>MSQSGEDLHSPTYLSWRKLQLSRAKLKASSKTSALLSGFAMVAMVEVQLDHDTNVPPGMLIAFAICTTLLVAVHMLALMISTCILPNIETVSNLHSISLVHESPHERLHWYIETAWAFSTLLGLILFLLEIAILCWV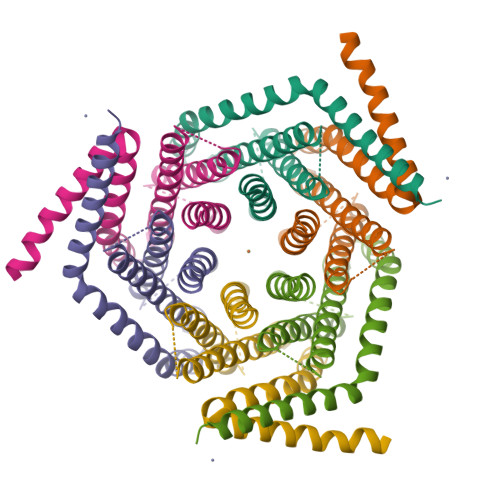KFYDLSRRAAWSATVVLIPVMIIFMAFAIHFYRSLVSHKYEVTVSGIRELEMLKEQMEQDHLEHHNNIRNNGEGEEF[2x]> GGSGPLKPEEHEDILNKLLDPELAQSERTEALQQLRVNYGSFVSEYNDLTKSHNTLSKELDNLRSRFGNLEGNTSERITIKNILQSRPDISAEECNFLMVEQIDSANLTTLQNTVKEIVLAVGIPYPKLRRKIPLLAIKLKYENIMLSNFAQRLH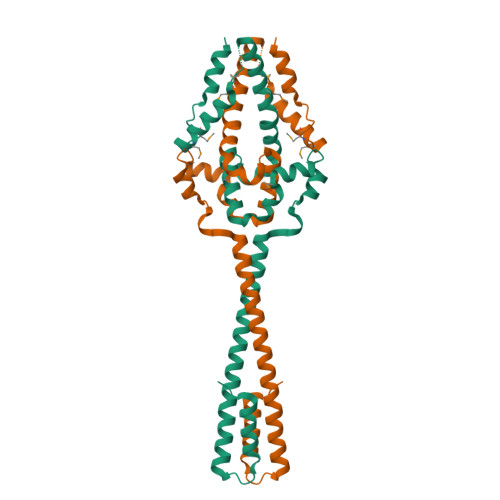RQVYSQEMNLKKFTDQAYYDFMSTRRMDSIDHHLERCLDHLYDHILEKMVK> NTDPEQCKVMCYAQ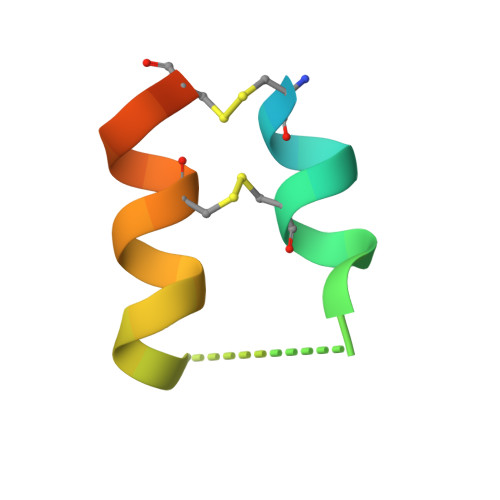RHSSPELLRRCLDNCEKEHD>[2x]MIKCSDVSNKIS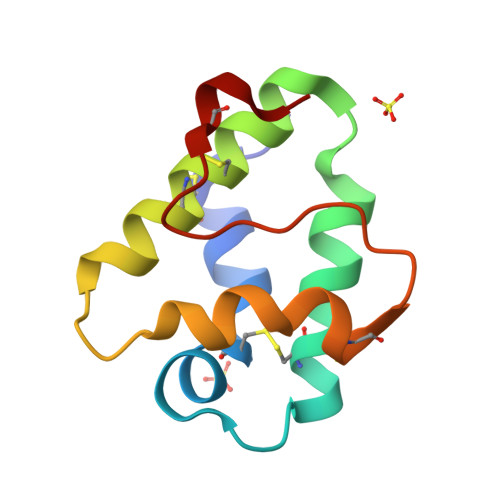ACLSYLKQGGEVPADCCTGVKGLNDAAKTTPDRQTACNCLKTTFKSNKDFKSDFAASLPSKCGVNIPYKISLETDCNKVK>[2x]TSDPVRQYLHEIGQVPLLTLEEEIDLARKVEEGMEAIKKLSEATGLDQELIREVVRAKILGTARIQKIPGLKEKPDPKTVE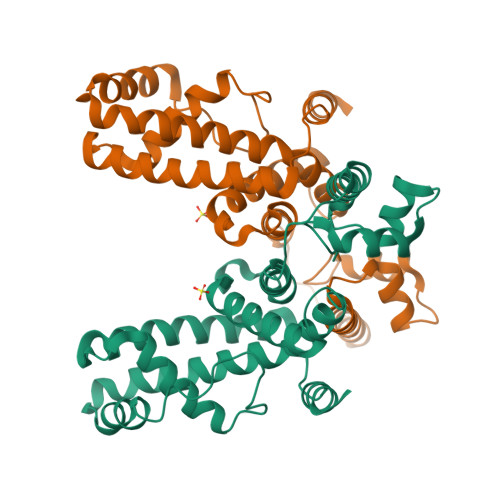EVDGKLKSLPKELKRYLHIAREGEAARQHLIEANLRLVVSIAKKYTGRGLSFLDLIQEGNQGLIRAVEKFEYKRRFKFSTYATWWIRQAINRAIADQARTIRIPVHMVETINKLSRTARQLQQELGREPSYEEIAEAMGPGWDAKRVEETLKIAQEPVSL> GAQRPRGPQRGKDIKHEISASLEELYKGRTAKLALNKQILCKECEGRGGKKGAVKKCTSCNGQGIKFVTRQMGPMIQRFQTECDVCHGTGDIIDPKDRCKSCNGKKVENERKILEVHVEPGMKDGQRIVFKGEADQAPDVIPGDVVFIVSERPH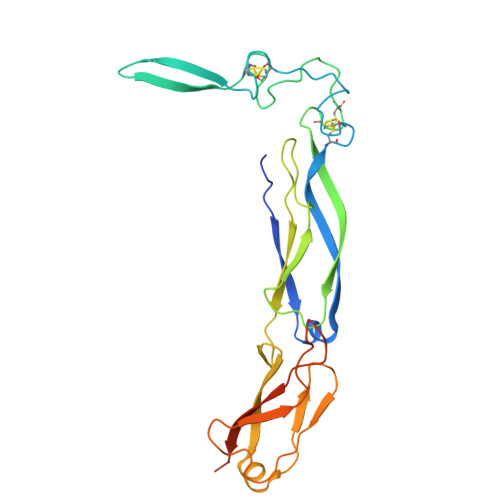KSFKRDGDDLVYEAEIDLLTAIAGGEFALEHVSGDWLKVGIVPGEVIAPGMRKVIEGKGMPIPKYGGYGNLIIKFTIKDPENHFTSEENLKKLE> MKSSHHHHHHENLYFQSNAALTTISPHDAQELIARGAKLIDIRDADEYLREHIPEADLAPLSVLEQSGLPAKLRHEQIIFHCQAGKRTSNNADKLAAIAAP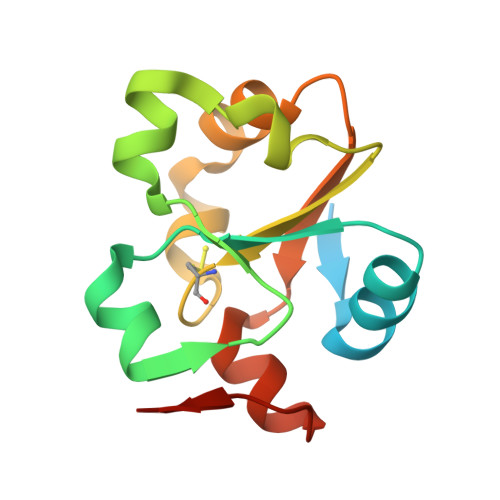AEIFLLEDGIDGWKKAGLPVAVNKSQ(4R)-4-(2-chloro-2,2-difluoroethyl)-1-{[(4R)-2-(methoxymethyl)-6-(trifluoromethyl)imidazo[2,1-b][1,3,4]thiadiazol-5-yl]methyl}pyrrolidin-2-one 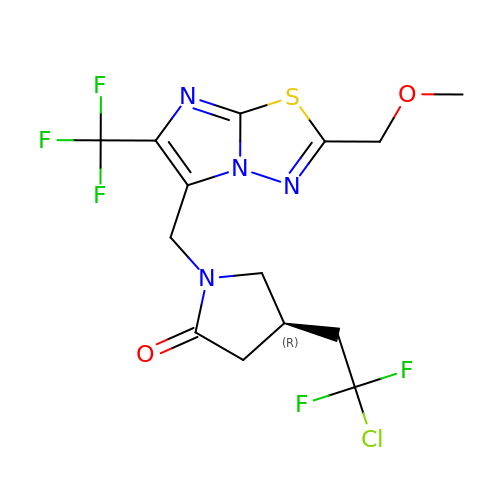| C14 H14 Cl F5 N4 O2 S | DCXFIOLWWRXEQH-SSDOTTSWSA-N>[2x]SMHEYAVGKIKIEHPWLRAPLEGETRAQLYMLVVNSADRPDRLIGVKSADFRSVQFHIAPHLVAREDAIYLPPLSRVTMAPGGSHVELVDISKMNPVGWAAEMTLVFEK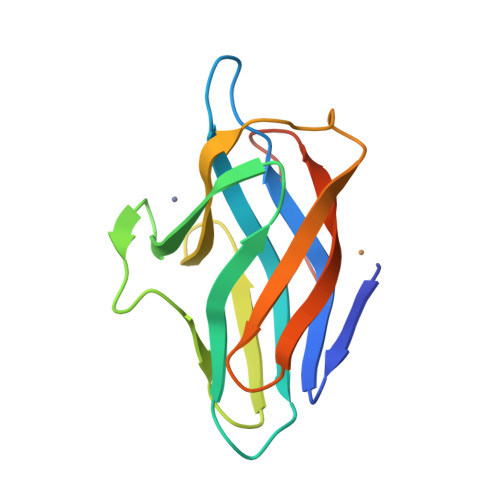AGEVTIDAAVEAPDAMHAHDAEAM>[2x]MEHAVIVENVTKKYKLFKRTSERLLDMILPGGYGEDFYALRNVSFTADKGDVIGIVGVNGSGKSTLSNIIAGILPPTSGTIKIDGQASLIAISSGLNNQLTGRENIELKCLMLGFSKKQIRAMEPDIIEFADIGKFIDQPVKTYSSGMKSRLGFAISVNIDPDVLVIDEALSVGDQTFADKCLDKMNEFKERGKTIFFISHS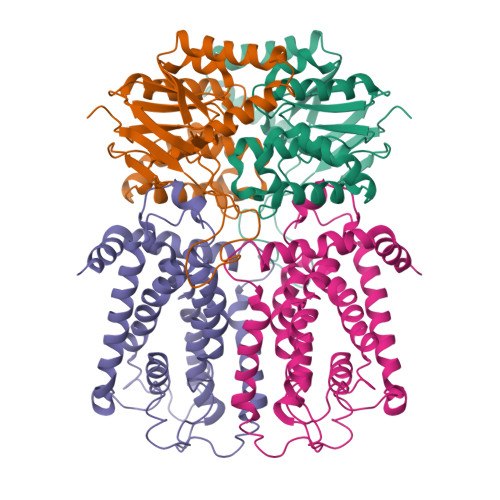IGQVKSFCEKALWLEYGEVRGYGTVAEIIPQYEKFLKEYRAMSDKEKRQYKERVMRKQQGEFLQAAVK;>MGHHHHHHHHHHMRSAVTVLMEHIRNLYLIRRLSLFELKSDNSNQYLGILWEIINPMIQIAIYWFVFGYGIRGRHPVGHIPFILWMLAGMTVWFFVNQAVLQASKSVYTRIRMVAQMNFPISVIPTYVITAKFYQHLMLLAVIFIIFQFTPYHVSVYLVQLPYYMFGLLALLVSFSLITSTLATVVRDVQMIVQSLVRILLYLTPLLWDPSHLPHLVQVIMRLNPLYYIVEGYRSALLGTSWYLVDHASYTVYFWVVVILFFVFGSMVHLKFRAHFVDYM[2x]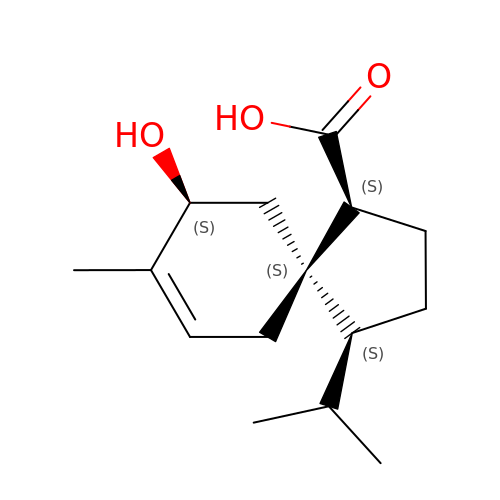(1S,4S,5S,9S)-9-hydroxy-8-methyl-4-(propan-2-yl)spiro[4.5]dec-7-ene-1-carboxylic acid | C15 H24 O3 | ZIOMQRRFPWLXDN-XFMPKHEZSA-N PII proteins are ubiquitous signaling proteins that are involved in the regulation of the nitrogen/carbon balance in bacteria, archaea, and some plants and algae. Signal transduction via PII proteins is modulated by effector molecules and post-translational modifications in the PII T-loop. In the present study, crystal structures of the PII protein GlnK from Corynebacterium glutamicum have been determined, namely of adenylylated GlnK (adGlnK) and unmodified unadenylylated GlnK (unGlnK). The allosteric signal that links effector binding to the regulation of the activity of PII-interacting proteins is primarily transduced via the T-loop, which adopts different conformations depending on the nature and combination of bound effectors.

The protein crystallized in the trigonal space group P32 and the final model contains six proteins chains per asymmetric unit. However, only three adenylyl moieties could be modeled with confidence in the adGlnK structure. Hence, only a single AMP moiety was modeled per two Tyr51 residues at each special position, namely the moiety that displayed the most easily interpretable electron density. This observation suggests that in the crystal, at any given point in time three adenylylated tyrosine residues are able to adopt defined conformations, while the other three residues are forced to adopt flexible conformations. While four of these sites appear to be devoid of any ligand, fortuitous binding of AMP and ADP was observed in the remaining two binding sites. In both the AMP- and ADP-binding sites, the adenine nucleobase is bound via two hydrogen bonds to the backbone of Ile64 from strand β3 and via one hydrogen bond to the side chain of Thr29 displayed from strand β2. Of the six T-loops present in the six PII monomers in the asymmetric unit of the adGlnK crystals, a considerably higher number of T-loop residues could be modeled in those loops in which the adenylylated Tyr51 residues are clearly resolved, and a considerably lower number of T-loop residues are visible in the two monomers where the effector-binding site is occupied by either AMP or ADP. In addition, the presence or absence of ligands, whether it be phosphate ions, AMP or ADP, appears to have little effect on the conformation of the T-loop in the present structures. This also holds true for the adenylylation of Tyr51, which also does not appear to affect the conformation of the T-loop. Interestingly, in both adenylylated GlnK and uridylylated GlnB, post-translational modification of the PII protein does not engender defined conformational rearrangements in the respective PII protein, hinting that complex formation is not modulated by an allosteric mechanism but that rather direct atomic interactions between the adenylylated Tyr51 of adGlnK and AmtR as well as between the uridylylated Tyr51 of GlnB and ATase promote complex formation.

>[6x]MKLITAIVKPFTLTDIKDALEQAGVQGMTVTETQGFGQQKGHTEVYRGAEYAVDFVPKVKIEVIISDAQAEEVINIIVETARTGKVGDGKVWMTNIEELVRVRTGERGEAAL To address these problems, a novel glycosyltransferase YojK from Bacillus subtilis 168 with the ability to glycosylate Reb A to produce Reb D was identified. To solve the solubility problem of plant-derived glycosyltransferases, YojK, a Leloir O-glycosyltransferase from B. subtilis 168, was selected to determine whether it had the catalytic ability to glycosylate Reb A to form Reb D, as it exhibits prominent glycosylation activity to various substrates like other bacterial glycosyltransferases with a large acceptor binding pocket. Then, the purified YojK was used to determine the glycosylation of Reb A. To our delight, it was found that Reb D was well synthesized by YojK with UDPG as the glycosyl donor, which was confirmed by LC-MS and NMR. Based on the catalytic mechanism of UDP-glycosyltransferases in the catalytic process, catalytic residue H14 of YojK firstly takes a proton from the hydroxyl group of the glucosyl unit at the C19-carboxylate position of Reb A to generate nucleophile, which then adopts SN2-like mechanism to attack the C1 carbon of the glucose of the sugar donor UDPG to form the β-1,2-linkage.

To better understand the molecular mechanism of YojK to catalyze the formation of Reb D from Reb A, we solved the crystal structure of YojK in complex with uridine diphosphate (UDP) and refined it to 1.90 Å solution. It consists of two monomers in each asymmetric unit. Similar to other bacterial glycosyltransferases, it folds a typical GT-B characteristic conformation containing two different β/α/β Rossmann domains connected by a variable loop region (V210-P224): a flexible N-domain (M1-F209) and a relatively rigid C-domain (F225-M405), which can be verified by superimposing the crystal structure of YojK with another bacterial glycosyltransferase YjiC. The flexible N-domain will allow YojK to accommodate various acceptor substrates, while the rigid C-domain contains a typical plant secondary product glycosyltransferase (PSPG) motif (Y288-Q329) with high conservation of sequence and structure, which is responsible for recognizing and binding the sugar donor. Similar to other glycosyltransferases, the catalytic site (H14-D107 catalytic triad at YojK) locates at the cleft region and closes to the center of the sugar donor and the acceptor substrate, and most of UDPG binding sites (except Y288 and D328) are highly conserved. However, the substrate binding pocket is highly plastic and flexible, and a large substrate binding pocket is observed in the crystal structure of YojK, indicating that it has an ability to accommodate diverse substrates, like the large substrate Reb A. With the crystal structure of YojK, we next performed structure-based engineering to improve its catalytic activity for the glycosylation of Reb A to produce Reb D. Probably due to low binding affinity between Reb A and YojK according to its enzymatic parameters, the crystal structure of YojK in complex with Reb A and UDPG was not obtained.

>MANVLMIGFPGEGHINPSIGVMKELKSRGENITYYAVKEYKEKITALDIEFREYHDFRGDYFGKNATGDEERDFTEMLCAFLKACKDIATHIYEEVKHESYDYVIYDHHLLAGKVIANMLKLPRFSLCTTFAMNEEFAKEMMGAYMKGSLEDSPHYESYQQLAETLNADFQAEIKKPFDVFLADGDLTIVFTSRGFQPLAEQFGERYVFVGPSITERAGNNDFPFDQIDNENVLFISMGTIFNNQKQFFNQCLEVCKDFDGKVVLSIGKHIKTSELNDIPENFIVRPYVPQLEILKRASLFVTHGGMNSTSEGLYFETPLVVIPMGGDQFVVADQVEKVGAGKVIKKEELSESLLKETIQEVMNNRSYAEKAKEIGQSLKAAGGSKKAADSILEAVKQKTQSANAALEHHHHHH[2x]>SQQLQKEEEARKVKSGIRQMRLFSQDECAKIEARIDEVVSRAEKGLYNEHTVDRAPLRNKYFFGEGYTYGAQLQKRGPGQERLYPPGDVDEIPEWVHQLVIQKLVEHRVIPEGFVNSAVINDYQPGGCIVSHVDPIHIFERPIVSVSFFSDSALCFGCKFQFKPIRVSEPVLSLPVRRGSVTVLSGYAADEITHCIRPQDIKERRAVIILRKTRLDAPRL[5x]

AlkB homologue 5 (ALKBH5) is a ferrous iron and 2-oxoglutarate dependent oxygenase that demethylates RNA N6-methyladenosine (m6A), a post-transcriptional RNA modification with an emerging set of regulatory roles. We report three crystal structures of ALKBH5 in complex with an m6A-ssRNA 8-mer substrate and supporting biochemical analyses. Strikingly, the single-stranded RNA substrate binds to the active site of ALKBH5 in a 5′-3′ orientation that is opposite to single-stranded or double-stranded DNA substrates observed for other AlkB subfamily members, including single-stranded DNA bound to FTO. The results support a mechanism involving formation of an m6A hemiaminal intermediate, followed by efficient ALKBH5 catalyzed demethylation, enabled by a proton shuttle network involving Lys132 and Tyr139.

Using higher ligand concentrations in the sample mixture and the crystallization drops, we subsequently determined structures of (i) ALKBH574–292 in complex with the same m6A-containing 8-mer ssRNA and the 2OG cosubstrate in the P32 crystal form to 2.1 Å resolution, and (ii) a structure of ALKBH574–292 in complex with NOG and the m6A-containing 8-mer ssRNA in the P21 crystal form to 2.5 Å resolution. The structure of the ALKBH574–292–NOG–RNA complex in space group P21 has five copies of the ALKBH574–292–NOG–ssRNA complex in the asymmetric unit, two of which manifest electron density for all eight nucleotides of the ssRNA substrate, likely in part due to stabilization by crystal packing contacts with neighboring molecules. Four (G−2G−1(m6A)0C+1) of the eight nucleotides are visible in the other three molecules in the asymmetric unit, in a similar manner for all the ssRNA substrate molecules in both the P32 crystal form structures. Aside from the four extra nucleotides observed in the P21 structure, the active site ssRNA binding modes in all the chains in the asymmetric units of the three structures are similar. At the ALKBH5 active site in the structures reported here, a catalytically inert Mn ion (substituting for catalytically active Fe(II)) is coordinated by the highly conserved metal binding triad His204, Asp206, and His266, a water molecule, and either 2OG, NOG, or a sulfate ion. In the structure of the ALKBH574–292–NOG–RNA complex, the NOG adopts a highly similar binding mode to 2OG, although with slight variations in the conformation of its C-5 carboxylate group. The crystallographically observed 2OG and NOG binding modes in ALKBH5 when complexed with Mn and an m6A substrate are of the ‘off-line’ mode. However, our crystallographic data may represent a snapshot of the complex in the catalytic process, where rearrangement of the 2OG C-1 carboxylate could occur.> PLTEQEIDELCDEWVPEPLIPPITEDMKHEPPVLESAAGPHTTVNGKDVVNFASANYLGLIGHEKLLESCTSALEKYGVGSCGPRGFYGTIDVHLDCETRISKFLGTPDSILYSYGLSTMFSTIPCFCKKGDVIVADEGVHWGIQNGLQLSRSTIVYFKHNDMESLRITLEKIMTKYKRSKNLRRYIVAEAVYQNSGQIAPLDEIVKLKEKYRFRVILDESNSFGVLGRSGRGLAEHHSVPIEKIDVVTAAMGHALATEGGFCTGNARIIDYQRLSSSGYVFSASLPPYLASAAITAIDVIDQNPDMLVKLKQNVALLWKGLSDIKGMSLTSNRESPIVFLKLEKSSGSAKDDLLLLEKMADRALKEDSLLVVSSKRSFLDKCRLPVGIKLYVSAGHSESDLLKASESLKRLASELLLKS;> MITIPYLTAVSTYFSYGLLFAFGQLRDFFRRFIDWWFTSNLQGYAPICLGHEDFYIRRLYHRIQDCFERPISSAPDAWFDVVERYSNDNNKTLKRTTKTSRCLNLGSYNYLGFGSFDEYCTPRVIESLKKFSASTCSSRVDAGTTSVHAELEECVTRFVGKPAAVVFGMGYATNSAIIPVLIGKGGLIISDSLNHSSIVNGARGSGATIRVFQHNTPSHLERVLREQIAEGQPRTHRPWKKIIVVVEGIYSMEGEICHLPEVVAICKKYKAYVYLDEAHSIGAIGKTGKGICELLGVDTADVDVMMGTFTKSFGSCGGYIAGSKELIQYLKHQCPAHLYATSIPTPSAQQIISAIKVILGEDGSNRGAQKLARIRENSNFFRAELQKMGFEVLGDNDSPVMPIMLYNPAKIPAFSRECLRQKVAVVVVGFPATPLLLARARICISASHSREDLIRALKVISKVGDLSGIKYFPAEPKKIEQSKNDIKLD;> MADYKDDDDKSGPDEVDASGRMNWVQRKIYLYNVTFGLYMLDWWERYLFNSLVVVLMWFVLYNGTRYFSELFQRHLT;> MANLYVKAVPPPDMNRNTEWFMYPGVWTTYMLILFFGWLVVLSVSGCSPGMAWTVVNLAHFVVTYHSFHWMKGTPFADDQGIYNGLTWWEQMDNGQQLTRNRKFLTLVPVVLYLIASHTTDYRHPWLFLNTLAVMVLVVAKFPNMHKVRIFGINGDK;> MASNLVEMFNAALNWVTMILESPSARVVLFGVPIRGHFFVEGLLGVVIIILLTRKSYKPPKR

The serine palmitoyltransferase (SPT) complex catalyzes the first and rate-limiting step in sphingolipid biosynthesis in all eukaryotes. ORM/ORMDL proteins are negative regulators of SPT that respond to cellular sphingolipid levels. We determined the cryo–electron microscopy structure of Arabidopsis SPT-ORM1 complex, composed of LCB1, LCB2a, SPTssa, and ORM1, in an inhibited state. The SPT-ORM1 complex is a ceramide sensor in the ER that controls cellular sphingolipid homeostasis.

During structural determination, a clear lipid-like density was observed in the cytosolic membrane leaflet sandwiched between ORM1 and LCB2a. The ceramide is presumably derived from endogenous ceramide copurifying with the SPT-ORM1 complex. The small polar head of C24-ceramide forms potential hydrogen bond interactions with the side-chain groups of Asn17 in ORM1 and Tyr55 in LCB2a and the main chain group of Ser67 in ORM1. The aliphatic sphingosine and acyl chains of ceramide are coordinated by numerous hydrophobic residues from both ORM1 and LCB2a. A hybrid β sheet, formed by the amino termini of ORM1 and LCB2a and induced by ceramide binding, stabilizes the amino terminus of ORM1 in an inhibitory conformation. Unlike either of these, the N terminus of AtORM1 (residues 5 to 8) forms an antiparallel hybrid β sheet with the N terminus of LCB2a (residues 1 to 5) in the AtSPT-ORM1 complex structure. The potential acyl-CoA binding pocket in the AtSPT-ORM1 structure is partially shielded by Met14 and Asn15 from ORM1. Our study demonstrates that upon ceramide binding, the N terminus of AtORM1 forms a hybrid β sheet with the N terminus of LCB2a, thus stabilizing the Met14/Asn15 of AtORM1 to limit acyl-CoA binding. The WT SPT-ORM1 complex represents a ceramide-bound state and has a decreased Vmax and an increased Khalf for palmitoyl-CoA compared to the ceramide-binding variant SPT-ORM1 (ORM1-N17A), indicating that the ceramide binding can repress SPT-ORM1 by mixed inhibition.> ADLDQGAQIFEAHCAGCHLNGGN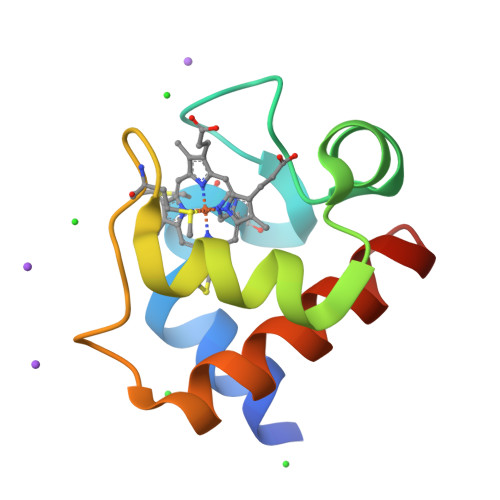IVRRGKNLKKRAMAKNGYTSVEAIANLVTQGKGNMSAYGDKLSSEEIQAVSQYVLQQSQTDWKS>GSQIHVDTMKVINDPIHGHIELHPLLVRIINTPQFQRLRYIKQLGGGYYVFPGASHNRFEHSLGVGYLAGCLVHALGEKQPELQISERDVLCVQIAGLCHDLGHGPFSHMFDGRFIPLARPEVKWTHEQGSVMMFEHLINSNGIKPVMEQYGLIPEEDICFIKEQIVGPLESPVEDSLWPYKGRPENKSFLYEIVSNKRNGIDVDKWDYFARDCHHLGIQNNFDYKRFIKFARVCEVDNELRICARDKEVGNLYDMFHTRNSLHRRAYQHKVGNIIDTMITDAFLKADDYIEITGAGGKKYRISTAIDDMEAYTKLTDNIFLEILYSTDPKLKDAREILKQIEYRNLFKYVGETQPTGQIKIKREDYESLPKEVASAKPKVLLDVKLKAEDFIVDVINMDYGMQEKNPIDHVSFYCKTAPNRAIRITKNQVSQLLPEKFAEQLIRVYCKKVDRKSLYAARQYFVQWCADRNFTKPQDGDVIAPLITPQKKEWNDSTSVQ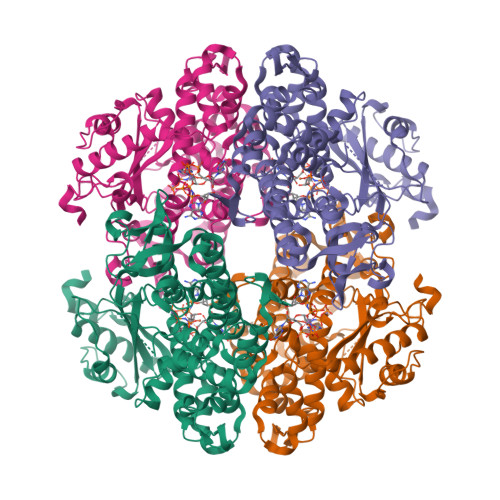NPTRLREASKSRVQLFKDDPM[2x]> MSAVALPRVSGGHDEHGHLEEFRTDPIGLMQRVRDELGDVGTFQLAGKQVVLLSGSHANEFFFRAGDDDLDQAKAYPFMTPIFGEGVVFDASPERRKEMLHNAALRGEQMKGHAATIEDQVRRMIADWGEAGEIDLLDFFAELTIYTSSACLIGKKFRDQLDGRFAKLYHELERGTDPLAYVDPYLPIESFRR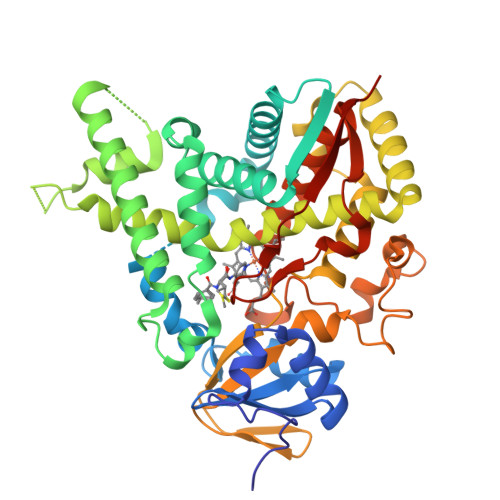RDEARNGLVALVADIMNGRIANPPTDKSDRDMLDVLIAVKAETGTPRFSADEITGMFISMMFAGHHTSSGTASWTLIELMRHRDAYAAVIDELDELYGDGRSVSFHALRQIPQLENVLKETLRLHPPLIILMRVAKGEFEVQGHRIHEGDLVAASPAISNRIPEDFPDPHDFVPARYEQPRQEDLLNRWTWIPFGAGRHRCVGAAFAIMQIKAIFSVLLREYEFEMAQPPESYRNDHSKMVVQLAQPAAVRYRRRTGVHHHH>[8x]MNDNVAWFKQAKYGMMIHWGLYSLLAGEYRGESSSAYAEWIQSKFQIPNAEYGNLATAFNPLYFDAKKIVALAKQCGMQYLVVTTKHHDGFAMYHSKVDAYNVYDATPFHRDIIGELAEACQKAGLKFGLYYSQDLDWHDPNGGGY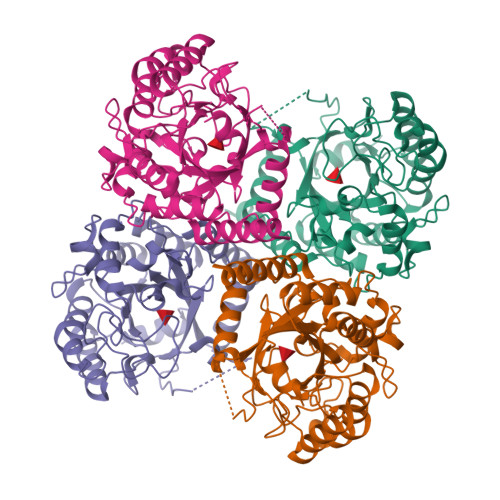KSNDVETAGTTWDNSWDFPDEDQKNFDLCFDNKILPQIKEIMSNYGDIATAWFDVPMTLSEAQSQTIYDTVRELQPNCLINSRLGNGKYDFVSLGDAEIPKNKEDMNKTDVDYNEITGFKPSPLGLYETAGTINDSWGFSYHDQNWKTPRTLYRYKQHLNDFGINYLLNVGLDPLGRVPMMAEENLLAAKALEDEANRL> MALISQSIKNLKGGISQQPDILRYPDQGSRQVNGWSSETEGLQKRPPLVFLNTLGDNGALGQAPYIHLINRDEHEQYYAVFTGSGIRVFDLSGNEKQVRYPNGSNYIKTANPRNDLRMVTVADYTFIVNRNVVAQKNTKSVNLPNYNPNQDGLINVRGGQ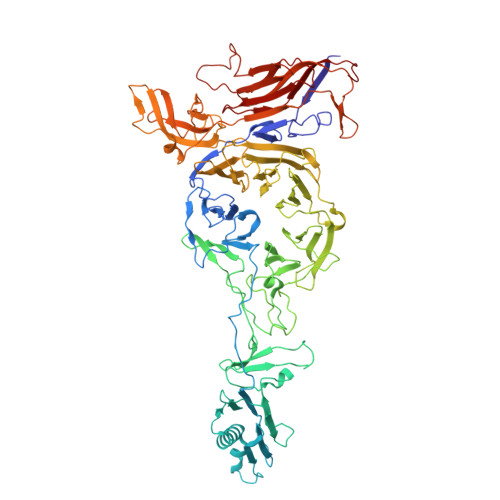YGRELIVHINGKDVAKYKIPDGSQPEHVNNTDAQWLAEELAKQMRTNLSDWTVNVGQGFIHVTAPSGQQIDSFTTKDGYADQLINPVTHYAQSFSKLPPNAPNGYMVKIVGDASKSADQYYVRYDAERKVWTETLGWNTEDQVLWETMPHALVRAADGNFDFKWLEWSPKSWGDVDTNPWPSFVGSSINDVFFFRNRLGFLSGENIILSRTAKYFNFYPASIANLSDDDPIDVAVSTNRIAILKYAVPFSEELLIWSDEAQFVLTASGTLTSKSVELNLTTQFDVQDRARPFGIGRNVYFASPRSSFTSIHRYYAVQDVSSVKNAEDITSHVPNYIPNGVFSICGSGTENFCSVLSHGDPSKIFMYKFLYLNEELRQQSWSHWDFGENVQVLACQSISSDMYVILRNEFNTFLARISFTKNAIDLQGEPYRAFMDMKIRYTIPSGTYNDDTFTTSIHIPTIYGANFGRGKITVLEPDGKITVFEQPTAGWNSDPWLRLSGNLEGRMVYIGFNINFVYEFSKFLIKQTADDGSTSTEDIGRLQLRRAWVNYENSGTFDIYVENQSSNWKYTMAGARLGSNTLRAGRLNLGTGQYRFPVVGNAKFNTVYILSDETTPLNIIGCGWEGNYLRRSSGI> MAMKNLLSLARRSQRRLFLTQATRSSSSFSAIDSVPASASPTALSPPPPHLMPY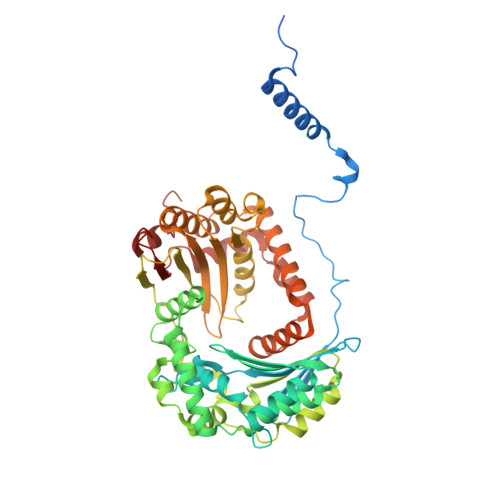DHAAEIIKNKIKKLENPDKRFLKYASPHPILASHNHILSAPETRVTTLPNGLRVATESNLSAKTATVGVWIDAGSRFESDETNGTAHFLEHMIFKGTDRRTVRALEEEIEDIGGHLNAYTSREQTTYYAKVLDSNVNQALDVLADILQNSKFEEQRINRERDVILREMQEVEGQTDEVVLDHLHATAFQYTPLGRTILGPAQNVKSITREDLQNYIKTHYTASRMVIAAAGAVKHEEVVEQVKKLFTKLSSDPTTTSQLVANEPASFTGSEVRMIDDDLPLAQFAVAFEGASWTDPDSVALMVMQTMLGSWNKNVGGGKHVGSDLTQRVAINEIAESIMAFNTNYKDTGLFGVYAVAKADCLDDLSYAIMYEVTKLAYRVSDADVTRARNQLKSSLLLHMDGTSPIAEDIGRQLLTYGRRIPTAELFARIDAVDASTVKRVANKYIYDKDIAISAIGPIQDLPDYNKFRRRTYWNRY>MARGVNKVILVGNVGGDPETRYMPNGNAVTNITLATSESWKDKQTGQQQERTEWHRVVFFGRLAEIAGEYLRKGSQVYVEGSLRTRKWQGQDGQDRYTTEIVV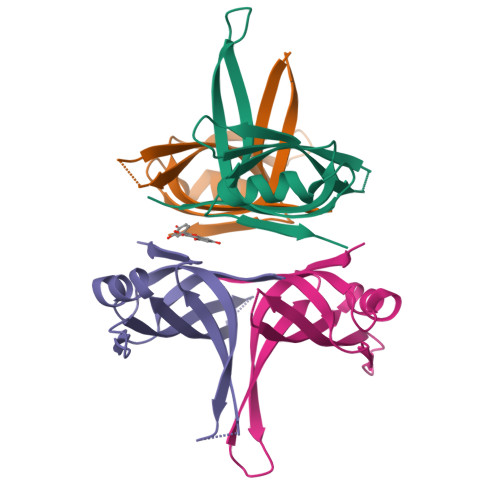DINGNMQLLGGRHHHHHH[4x]> SGTTNTVAAYNLTWKSTNFKTILEWEPKPVNQVYTVQISTKSGDWKSKCFYTTDTECDLTD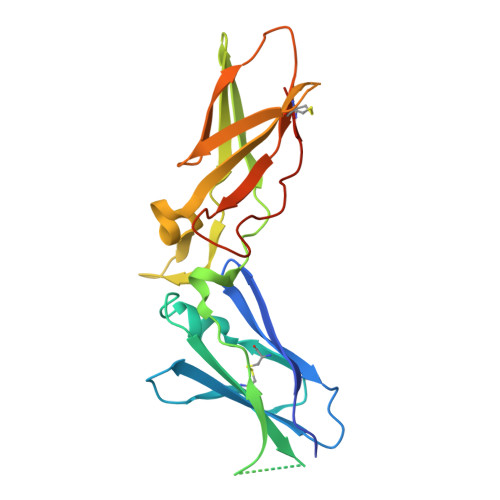EIVKDVKQTYLARVFSYPAGNVESTGSAGEPLYENSPEFTPYLETNLGQPTIQSFEQVGTKVNVTVEDERTLVRRNNTFLSLRDVFGKDLIYTLYYWKSSSSGKKTAKTNTNEFLIDVDKGENYCFSVQAVIPSRTVNRKSTDSPVECMGQEKGEFR> NPASPPEEGSPDPDSTGALVEEEDPFFKVPVNKLAAAVSNFGYDLYRVRSSTSPTTNVLLSPLSVATALSALSLGAEQRTESIIHRALYYDLISSPDIHGTYKELLDTVTAPQKNLKSASRIVFEKKLRIKSSFVAPLEKSYGTRPRVLTGNPRLDLQEINNWVQAQMKGKLARSTKEIPDEISILLLGVAHFKGQWVTKFDSRKTSLEDFYLDEERTVRVPMMSDPKAVLRYGLDSDLSCKIAQLPLTGSMSIIFFLPLKVTQNLTLIEESLTSEFIHDIDRELKTVQAVLTVPKLKLSYEGEVTKSLQEMKLQSLFDSPDFSKITGKPIKLTQVEHRAGFEWNEDGAGTTPSPGLQPAHLTFPLDYHLNQPFIFVLRDTDTGALLFIGKILDPRGP

However, PEDF lacks a consensus sequence for the serpin reactive center region and exhibits no antiprotease activity, while being a major neurotrophic factor in the retina that promotes neurogenesis and enhances the viability of photoreceptors, amacrine cells, and other neurons. Interestingly, PEDF belongs to the serpins (SERPINF1), a family of serine proteinase inhibitors other members of which have also been identified as zinc-binding proteins, suggesting that zinc coordination is a common property of this family and may affect ocular proteostasis. PEDF acts through the interaction with cell surface receptors, mainly PEDF-R, which contribute significantly to the survival of retinal cells. Biophysical and X-ray crystallographic studies show that PEDF coordinates zinc ions in five types of intermolecular high-affinity sites, leading to a decrease in negative surface charge and reversible oligomerization of the protein, thereby masking the target recognition sites responsible for its neurotrophic and antiangiogenic activities and collagen binding.

To identify all the zinc coordination sites, we next crystallized PEDF in the presence of this metal and collected X-ray diffraction data. Crystals were obtained in two space groups, P21212 and P212121, with one and five protein molecules in the asymmetric unit. In both cases, the crystals gave diffraction data up to ~2 Å. Zinc binding sites were identified in both space groups: 1 site for P21212 and 7 sites for P212121. Importantly, all identified sites were located at the intermolecular interfaces and included coordinators from two or three protein molecules confirming the role of zinc as a promoter of PEDF oligomerization observed in DLS studies. The type 1 site, which was also predicted by ZincBind appears to be the strongest and most important, and its occupancy seems to affect the properties of PEDF at low zinc concentrations. Indeed, PEDF-R binding and neurotrophic activity of PEDF have been shown to be provided by its 44-mer fragment spanning amino acid residues at positions 78–12170,83–85. According to our structural analysis, zinc binding to sites of types 1, 4 and 5 results in this fragment localizing at the intermolecular interface of the resulting dimer/trimer, impeding its access to the receptor. Zinc concentration corresponding to filling the high-affinity site in PEDF (4 μM) matches the level of elevated zinc in AH of some patients with POAG (2–7 μM), suggesting that this metal is unlikely to bind to PEDF under normal conditions (0.4–0.5 μM Zn2+) but may be captured under pathologic conditions.> GAACGACACTGA;> CGTGGACTC;> TCAACG;> TCGA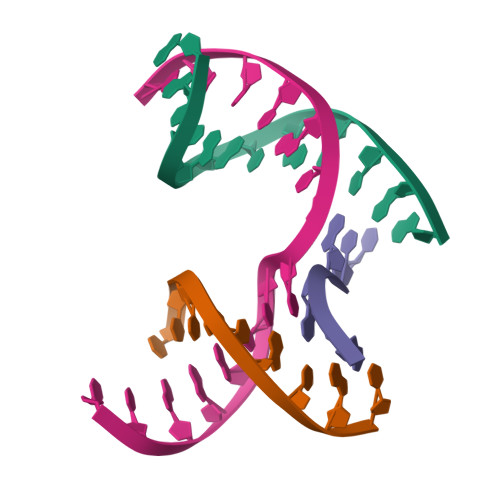GTCCGTGTCGT Protein arginine methyltransferases (PRMTs) are important therapeutic targets, playing a crucial role in the regulation of many cellular processes and being linked to many diseases. Then, another series of compounds (12a–12h) were designed and synthesized, introducing also an adenosine moiety and exploring the distance between the three groups. We also report crystal structures with various PRMTs supporting the observed specificity and selectivity. On the contrary, we were able to cocrystallize the compounds in the complex with both PRMT4 and PRMT6.

Structure determinations and refinements revealed that only compounds 12a, 12c, and 12f are visible in the active site of each monomer of the PRMT6 dimer. Compound 12a is the only one for which a complete electron density is visible in one monomer of the PRMT6 structure, whereas for 12c and 12f the electron density becomes fragmented after the guanidine group and the density for the methyl-4-hydroxy-2-naphthoate moiety is weak. The crystal structure revealed an unusual distorted U-shaped conformation adopted by compound 12a (and probably also 12c and 12f) in the binding to PRMT6, with a folding at the level of the guanidine group. Whereas the adenosine moiety lies into its canonic binding pocket, the guanidine group of the compounds is unable to reach the PRMT6 double-E loop clamp because the linker with the sugar is too short, even for the longer compound 12f. Instead of binding in the arginine substrate pocket as observed with PRMT4, the methyl-4 hydroxy-2-naphthoate moiety is sandwiched between the adenosine and the side chains of Y50 and Y51 residues of the α helix motif I. Hence, the binding of compounds 12a, 12c, and 12f affects the proper folding of the PRMT6 alpha-X helix containing the motif I (Y50-Y51-X-X-Y54). If compared to the structures obtained in the presence of SAH, the binding site of the complex of PRMT6 with compound 12a is larger due to a displacement of the α helix and the flipping of the side chains of Y50 and Y51 residues to give room for the compound naphthoate moiety. As a consequence, the E267 residue of the double-E loop is not coordinated anymore by residues Y50 and Y54 of motif 1 and adopts a different conformation.

>[2x]MSLSKKRKLESGDSGGAGAGGEGAEEENGGEQEAAPPRPRRTKSERDQLYYECYSDVSVHEEMIADQVRTEAYRLGILKNWAALRGKTVLDVGAGTGILSIFCAQAGARRVYAVEASAIWQQAREVVRLNGLEDRVHVLPGPVETVELPERVDAIVSEWMGYGLLHESMLSSVLHARTKWLKEGGLLLPASAELFVAPISDQMLEWRLGFWSQVKQHYGVDMSCMESFATRCLMGHSEIVVQDLSGEDVLARPQRFAQLELARAGLEQELEAGVGGRFRCSCYGSAPLHGFAVWFQVTFPGGDSEKPLVLSTSPLHPATHWKQALLYLNEPVPVEQDTDISGEITLLPSPDNPRRLRILLRYKVGDHEEKTKDFAMEDGSENLYFQ(C8-S)-HYDANTOCIDIN 5'-PHOSPHATE | C13 H22 N3 O13 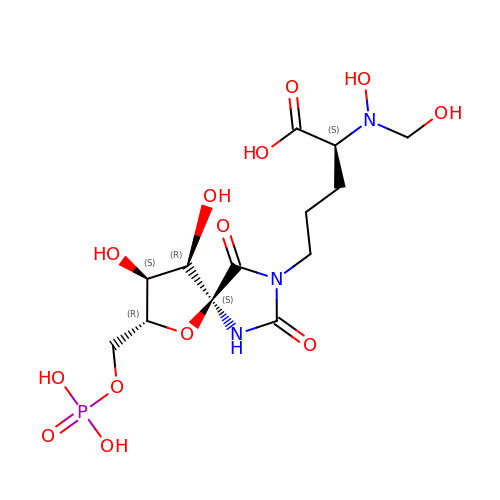P | MAXSFYCTFIBEAR-FUIMDIGMSA-N> MKVGQDKVVTIRYTLQVEGEVLDQGELSYLHGHRNLIPGLEEALEGREEGEAFQAHVPAEKAYGPHDPEGVQVVPLSAFPEDAEVVPGAQFYAQDMEGNPMPLTVVAVEGEEVTVDFNHPLAGKDLDFQVEVVKVREATPEELLHGHAHPSGHHHHHH;>VGSN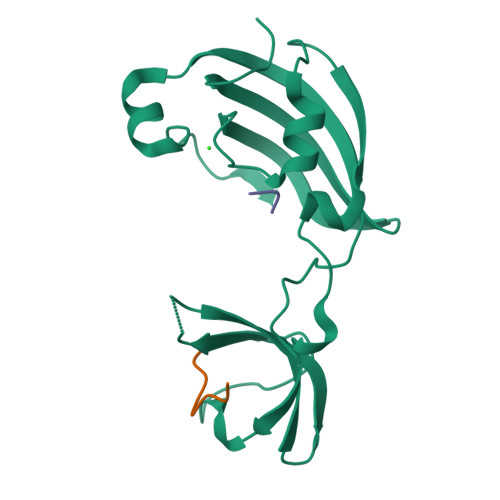SYPHKYNNYEGX[2x]>[12x]HHHHHHSEMTPREIVSELDKHIIGQDNAKRSVAIALRNRWRRMQLNEELRHEVTPKNILMIGPTGVGKTEIARRLAKLANAPFIKVEATKFTEVGYVGKEVDSIIRDLTDAAVKMVRVQAIEKNRYRAEELAEERILDVLIPPAKNNWGQTEQQQEPSAARQAFRKKLREGQLDDKEIEIDLAAAPMGVEIMAPPGMEEMTSQLQSMFQNLGGQKQKARKLKIKDAMKLLIEEEAAKLVNPEELKQDAIDAVEQHGIVFIDEIDKICKRGESSGPDVSREGVQRDLLPLVEGCTVSTKHGMVKTDHILFIASGAFQIAKPSDLIPELQGRLPIRVELQALTTSDFERILTEPNASITVQYKALMATEGVNIEFTDSGIKRIAEAAWQVNESTENIGARRLHTVLERLMEEISYDASDLSGQNITIDADYVSKHLDALVADEDLSRFIL

HslUV consists of one or two AAA+ HslU6 ring hexamers and the double-ring HslV12 peptidase (Rohrwild et al., 1997; Sousa et al., 2000; Wang et al., 2001). ATP-dependent proteolysis requires HslU6 to bind the degrons of target proteins in its axial channel and then unfold and translocate the substrate into the proteolytic chamber of HslV12. To reach the axial channel of the HslU hexamer, substrates must transit a funnel-like structure formed by segments of its intermediate (I) domain (Sousa et al., 2000; Wang et al., 2001). Here, we present evidence for a model in which HslU hexamers are autoinhibited at low temperatures by a trimeric I-domain plug that blocks the axial channel but melts at high temperatures to activate proteolysis.

We determined structures for three new crystal forms of E. coli HslU or HslUV by molecular replacement. Our new structures were similar to previous ones with the notable exception that a trimeric plug, formed by residues 183–206 of the I-domain, completely blocked the axial channel of the HslU ring. The plug consisted of amino acids from three of the six HslU subunits, each comprising an extended region (residues 183–188), a sharp turn (residues 189–191), and an α helix (residues 192–206). We could not reliably model connections between plug elements and other regions of the I-domain in specific subunits. The three α helices that comprise the plug center packed together via hydrophobic contacts involving the side chains of Met192, Met195, Leu199, and Phe203. Additional hydrophobic packing contacts within the plug included Val184 and Ile186 from the extended region, which occupy peripheral grooves between plug helices, and Met202 from the helix. A Pro189-Pro190-Gly191 tripeptide formed a sharp turn between the extended region and α helix of the plug. The negatively charged side chains of Glu193 and Glu194 following this turn were also close to the positively charged side chains of Arg101 (94% conserved) and Lys293 (92% conserved) in the HslU axial channel, suggesting that favorable electrostatic interactions also stabilize the plugged conformation. Because protein substrates must access the axial channel of HslU to be engaged, unfolded, and translocated into the peptidase chamber of HslV, this plug would inhibit substrate degradation. Hence, replacing the nonpolar Leu199 with a polar Gln199 in the L199QHslU variant should destabilize helix-helix packing and plug stability, thereby reducing autoinhibition and providing a structural rationale for the ability of L199QHslUV to degrade some protein substrates more rapidly than wild-type HslUV (WTHslUV; Baytshtok et al., 2016).>MCIIFFKFDPRPVSKNAYRLILAANRDEFYSRPSKLADFWGNNNEILSGLDMEEGKEGGTWLGISTRGKLAALTNYLQPQLDWQARGRGELVTHFLTTDVDSLSYLKKVSMEGHLYNGFNLIAADLSTAKGDVICYYGNRGEPDPIVLTPGTYGLSNALLETPWRKLCFGKQLFLEAVERSQALPKDVLIA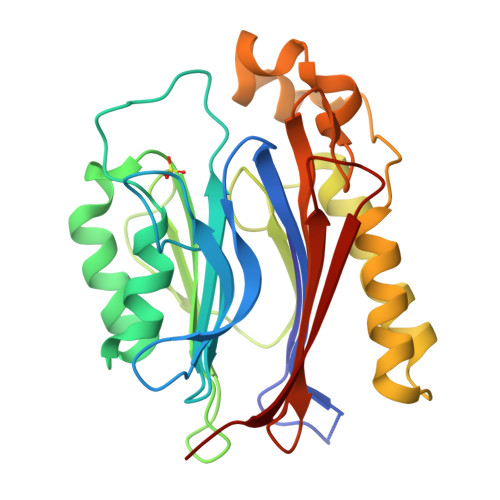SLLDVLNNEEAQLPDPAIEDQGGEYVQPMLSKYAAVCVRCPGYGTRTNTIILVDADGHVTFTERSMMDKDLSHWETRTYEFTLQS[2x]> GSMEDVEIKPRGYQLRLVDHLTKSNGIVYLPTGSGKTFVAILVLKRFSQDFDKPIESGGKRALFMCNTVELARQQAMAVRRCTNFKVGFYVGEQGVDDWTRGMWSDEIKKNQVLVGTAQVFLDMVTQTYVALSSLSVVIIDECH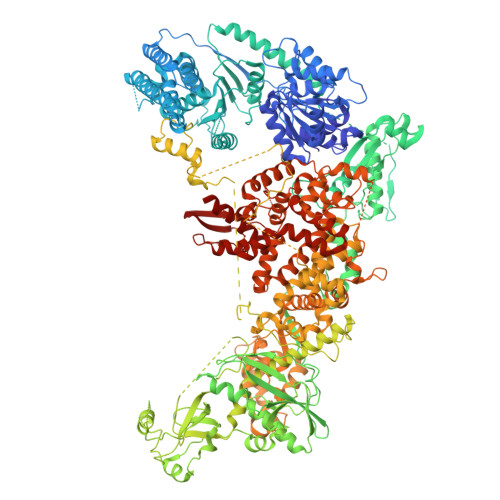HGTGHHPFREFMRLFTIANQTKLPRVVGLTGVLIKGNEITNVATKLKELEITYRGNIITVSDTKELENVMLYATKPTEVMVSFPHQEQVLTVTRLISAEIEKFYVSLDLMNIGVQPIRRSKSLQCLRDPSKKSFVKQLFNDFLYQMKEYGIYAASIAIISLIVEFDIKRRQAETLSVKLMHRTALTLCEKIRHLLVQKLQDMTYDDDDDNVNTEEVIMNFSTPKVQRFLMSLKVSFADKDPKDICCLVFVERRYTCKCIYGLLLNYIQSTPELRNVLTPQFMVGRNNISPDFESVLERKWQKSAIQQFRDGNANLMICSSVLEEGIDVQACNHVFILDPVKTFNMYVQSKGRARTTEAKFVLFTADKEREKTIQQIYQYRKAHNDIAEYLKDRVLEKTEPELYEIKGHFQDDIDPFTNENGAVLLPNNALAILHRYCQTIPTDAFGFVIPWFHVLQEDERDRIFGVSAKGKHVISINMPVNCMLRDTIYSDPMDNVKTAKISAAFKACKVLYSLGELNERFVPKTLKERVASIADVHFEHWNKYGDSVTATVNKADKSKDRTYKTECPLEFYDALPRVGEICYAYEIFLEPQFESCEYTEHMYLNLQTPRNYAILLRNKLPRLAEMPLFSNQGKLHVRVANAPLEVIIQNSEQLELLHQFHGMVFRDILKIWHPFFVLDRRSKENSYLVVPLILGAGEQKCFDWELMTNFRRLPQSHGSNVQQREQQPAPRPEDFEGKIVTQWYANYDKPMLVTKVHRELTPLSYMEKNQQDKTYYEFTMSKYGNRIGDVVHKDKFMIEVRDLTEQLTFYVHNRGKFNAKSKAKMKVILIPELCFNFNFPGDLWLKLIFLPSILNRMYFLLHAEALRKRFNTYLNLHLLPFNGTDYMPRPLEIDYSLKRNVDPLGNVIPTEDIEEPKSLLEPMPTKSIEASVANLEITEFENPWQKYMEPVDLSRNLLSTYPVELDYYYHFSVGNVCEMNEMDFEDKEYWAKNQFHMPTGNIYGNRTPAKTNANVPALMPSKPTVRGKVKPLLILQKTVSKEHITPAEQGEFLAAITASSAADVFDMERLEILGDSFLKLSATLYLASKYSDWNEGTLTEVKSKLVSNRNLLFCLIDADIPKTLNTIQFTPRYTWLPPGISLPHNVLALWRENPEFAKIIGPHNLRDLALGDEESLVKGNCSDINYNRFVEGCRANGQSFYAGADFSSEVNFCVGLVTIPNKVIADTLEALLGVIVKNYGLQHAFKMLEYFKICRADIDKPLTQLLNLELGGKKMRANVNTTEIDGFLINHYYLEKNLGYTFKDRRYLLQALTHPSYPTNRITGSYQELEFIGDAILDFLISAYIFENNTKMNPGALTDLRSALVNNTTLACICVRHRLHFFILAENAKLSEIISKFVNFQESQGHRVTNYVRILLEEADVQPTPLDLDDELDMTELPHANKCISQEAEKGVPPKGEFNMSTNVDVPKALGDVLEALIAAVYLDCRDLQRTWEVIFNLFEPELQEFTRKVPINHIRQLVEHKHAKPVFSSPIVEGETVMVSCQFTCMEKTIKVYGFGSNKDQAKLSAAKHALQQLSKCDA(5~{S})-1-(3-chloranyl-4-methoxy-phenyl)-5-[4-(3-methyl-1,2-benzoxazol-5-yl)-1-[(2~{R})-2-morpholin-4-ylpropyl]imidazol-2-yl]pyrrolidin-2-one 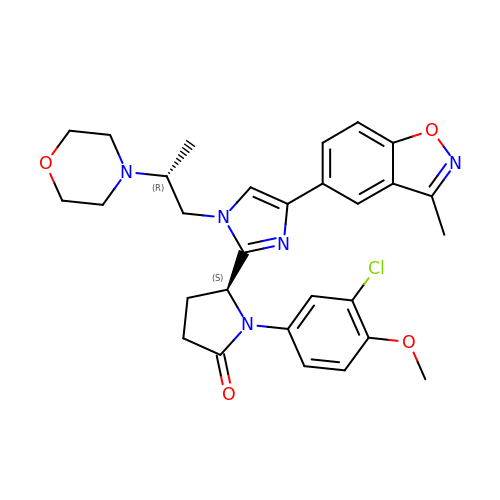| C29 H32 Cl N5 O4 | KUECYLYQFQZBBX-CJAUYULYSA-N> MRGSHHHHHHGLVPRGSMIRTMLQGKLHRVKVTHADLHYEGSCAIDQDFLDAAGILENEAIDIWNVTNGKRFSVYAIAAERGSRIISVNGAAAHCASVGDIVIIASFVTMPDEEARTWRPNVAYFEGDNEMKRTAKAIPVQVA;> MKLTIIRLEKFSDQDRIDLQKIWPEYSPSSLQVDDNHRIYAARFNERLLAAVRVTLSGTEGALDSLRVREVTRRRG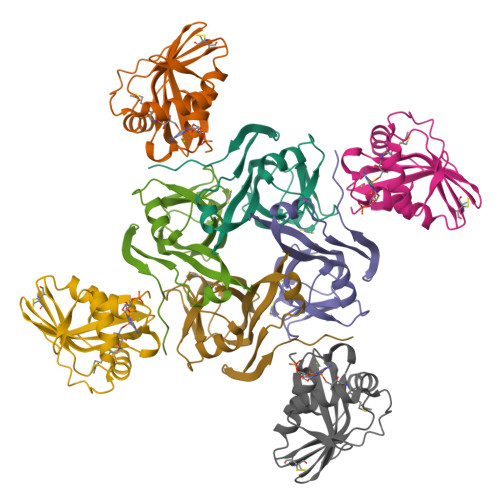VGQYLLEEVLRNNPGVSCWWMADAGVEDRGVMTAFMQALGFTAQQGGWEKCSGLEHHHHHH The template for transcription is a complex between the viral RNA and the nucleoprotein (NP) that binds to the RNA sugar-phosphate backbone. NP is necessary for RNA elongation by the polymerase. The formation of such complexes results from two coupled activities of the nucleoproteins: RNA binding and self polymerisation. The nucleoproteins of influenza A H1N1 and H5N1 crystallised as trimers and NP of influenza B virus as a tetramer.

We then crystallised the obligate monomeric R416A mutant of NP. Crystals with space group C2221 diffracted to 2.7 Å. Even though the crystals of wt and mutant NP have the same space group, wt NP crystallises as a trimer whereas mutant NP crystallised as a monomer but with 3 molecules in the asymmetric unit; the cell dimensions are different and the positions of the monomers are different from those of the protomers in the trimer. Most of the mutant protein structure is identical to that of the wt, from residue 22 to 385, the rmsd is 1.09 Å for 364 aligned Cα's. From residue 386 onward the structure is different because the exchange domain folds into the groove of its own protomer rather than in the groove of a neighbouring protomer. In the monomeric mutant protein, residues 386–390 form a β-strand (β7) and residues 392–407 form a flexible loop that points towards the RNA binding surface. For trimeric H1N1 the last visible C-terminal residue is 489 and for H5N1 this is residue 496 and in both structures the C-termini point away from the RNA binding surface. However, in the structure of R416A, the chain is visible until the penultimate residue and points into the RNA binding surface, reducing the space for RNA binding and changing the electrostatic characteristics of this surface (compare figures 3C, F and I, blue is positively charged). In the R416A structure, E339 makes hydrogen bonds with R461 and the mutated R416A points towards R461; if the wt monomer structure were the same as the R416A structure there could be a clash between arginines 416 and 461. Therefore, the R416A mutation may both stabilise the monomer and destabilise the trimer. The structure of the monomer can perhaps best be described as self-inhibited in which the exchange domain that is involved in trimer formation takes up equivalent positions on its own core rather than on the core of a neighbouring protomer.

>[3x]MATKGTKRSYEQMETDGERQNATEIRASVGKMIDGIGRFYIQMCTELKLSDYEGRLIQNSLTIERMVLSAFDERRNKYLEEHPSAGKDPKKTGGPIYRRVDGKWRRELILYDKEEIRRIWRQANNGDDATAGLTHMMIWHSNLNDATYQRTRALVRTGMDPRMCSLMQGSTLPRRSGAAGAAVKGVGTMVMELIRMIKRGINDRNFWRGENGRRTRIAYERMCNILKGKFQTAAQRTMVDQVRESRNPGNAEFEDLIFLARSALILRGSVAHKSCLPACVYGSAVASGYDFEREGYSLVGIDPFRLLQNSQVYSLIRPNENPAHKSQLVWMACHSAAFEDLRVSSFIRGTKVVPRGKLSTRGVQIASNENMETMESSTLELRSRYWAIRTRSGGNTNQQRASSGQISIQPTFSVQANLPFDRPTIMAAFTGNTEGRTSDMRTEIIRLMESARPEDVSFQGRGVFELSDEKATSPIVPSFDMSNEGSYFFGDNAEEYDN> GPEIIKWQPHQQNKWATLY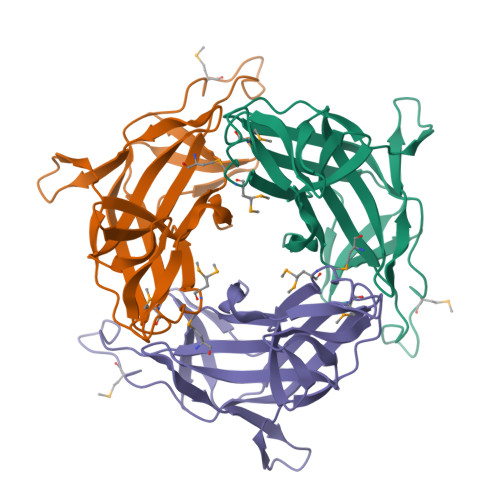DANYKELPMLTYRVDADKGFNFSVGDDAFVCQKKNHFQVTVYIGMLGEPKYVKTPEGLKPLDCFYLKLHGVKLEALNQSINIEQSQSDRSKRPFNPVTVNLPPEQVTKVTVGRLHFSETTANNMRKKGKPNPDQRYFMLVVALQAHAQNQNYTLAAQISERIIVRAS>MDKLPPSMRKRLYSLPQQVGAKAWIMDEEEDAEEEGAGGRQDPRRRSIRLRPLPSPSPSPSAAAAAAGGAESRGAALGGAADGEGPARGAAKSSTNGDCRRFRGSLASLGSRGGGGGGGSTGGGSHGHLHDSAEERRLIAEGDASPGEDRTPPGLAAEPERPGAPAPPAASPPQVPSSCGEQRPADAAVKVEGGAAAGDQIL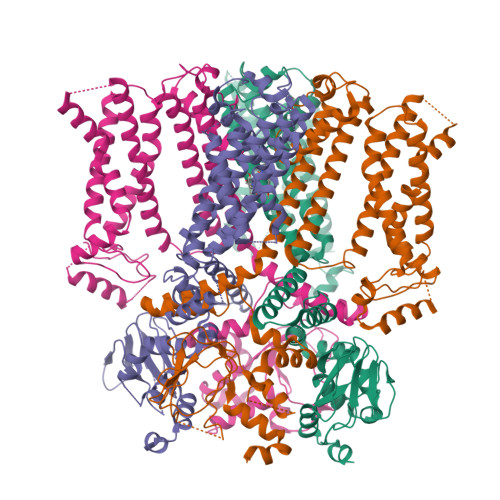PEAEARLGQAGFMQRQFGAMLQPGVNKFSLRMFGSQKAVEREQERVKSAGFWIIHPYSDFRFYWDLTMLLLMVGNLIIIPVGITFFKDENTTPWIVFNVVSDTFFLIDLVLNFRTGIVVEDNTDIILDPRRIKMKYLKSWFVVDFVSSIPVDYIFLIVETRIDSEVYKTARALRIVRFTKILSLLRLLRLSRLIRYIHQWEEIFHMTYDLASAVVRIVNLIGMMLLLCHWDGCLQFLVPMLQDFPDDCWVSLNNMVNNSWGKQYSYALFKAMSHMLCIGYGRQAPMGMSDVWLTMLSMIVGATCYAMFIGHATALIQSLDSSRRQYQEKYKQVEQYMSFHKLPPDTRQRIHDYYEHRYQGKMFDEESILGELSEPLREEIINFNCRKLVASMPLFANADPNFVTSMLTKLRFEVFQPGDYIIREGTIGKKMYFIQHGVVSVLTKGNKETKLADGSYFGEICLLTRGRRTASVRADTYCRLYSLSVDNFNEVLEEYPMMRRAFETVALDRLDRIGKKNSIHKVQHDLSSGVSNYQENAIVQRIVQHDREMAHCARRAQATTPVAPAIWTPLIQAPLQAAAQDLKLISASQPALPQDGAQTLRRASPHSSSGESVAALPPAGGPFPRAPGRPPGAGPGQHVTLTLPRKASSGSLPPPLSLFGPRAAPRLTAAPQREPGAKSEPVRSKLPSNL[4x]> MGSMVKLDRYIGVTVFVAILAVLGVILGLALLFAFIDEL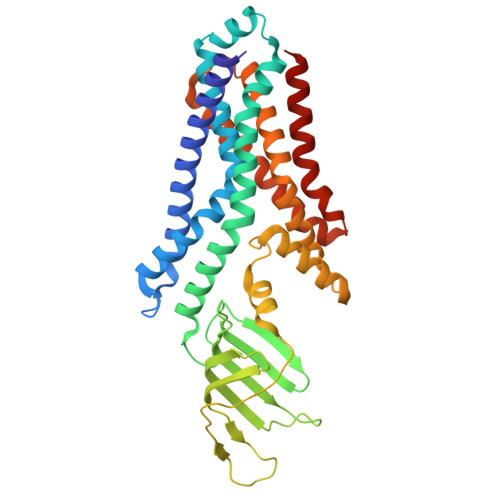NDISASYGIGDALRFIFLTAPRRAYDMLPMAALIGCLVGLGTLASNSELTIMRAAGVSLSRIVWAVMKPMLVLMLAGILVGEYVAPWTENIAQSGRALAQGGGDSQSSKRGLWHRQGREYIHINAVQPNGVLYGVTRYRFDEQRGLESASFAKRARFETDHWQLEEVTTTLLHPREKRSEVVKLPTERWDAQLSPQLLNTVVMEPEALSISGLWQYIHYLADQGLNNNRYWLAFWTKVLQPLVTAALVLMAISFIFGPLRSVTLGQRIFTGVLVGFVFRIAQDLLGPSSLVFDFPPLLAVVIPASICALAGVWLLRRAG>[3x]MSSKP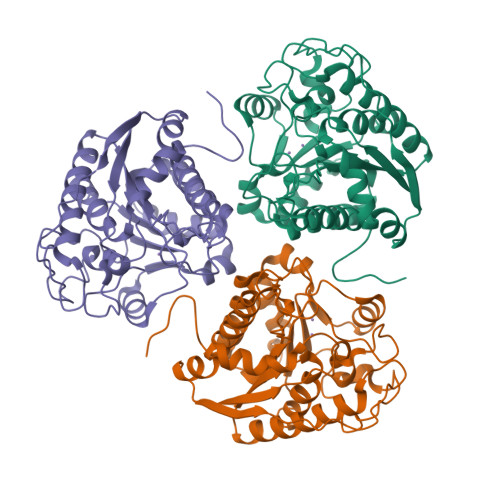KPIEIIGAPFSKGQPRGGVEKGPAALRKAGLVEKLKETEYNVRDHGDLAFVDVPNDSPFQIVKNPRSVGKANEQLAAVVAETQKNGTISVVLGGDHSMAIGSISGHARVHPDLCVIWVDAHTDIATPLTTSSGNLHGQPVAFLLKELKGKFPDVPGFSWVTPCISAKDIVYIGLRDVDPGEHYIIKTLGIKYFSMTEVDKLGIGKVMEETFSYLLGRKKRPIHLSFDVDGLDPVFTPATGTPVVGGLSYREGLYITEEIYKTGLLSGLDIMEVNPTLGKTPEEVTRTVNTAVALTLSCFGTKREGNHKPETDYLKPPK> VKPISPEQEELIHRLVYFQNEYEQPSDEDLKRISNTPSEGEDQSDLNFRHITEITILTVQLIVEFAKRLPGFDKLLREDQIALLKACSSEVMMLRMARRYDVGSDSILFANNQPYTRDSYSLAGMGETVDDLLRFCRQMYGMKVDNAEYALLTAIVIFSERPSLIEGWKVEKIQEIYLEALKVYVDNRRKPASGTIFAKLLSVLTELRTLGNLNSEMCFSLKLKNKKLPPFLAEIWDV;> NAVANICQATNSQLYQLVEWAKHIPHFSSLPIEDQVLLLRAGWNELLIAAFSH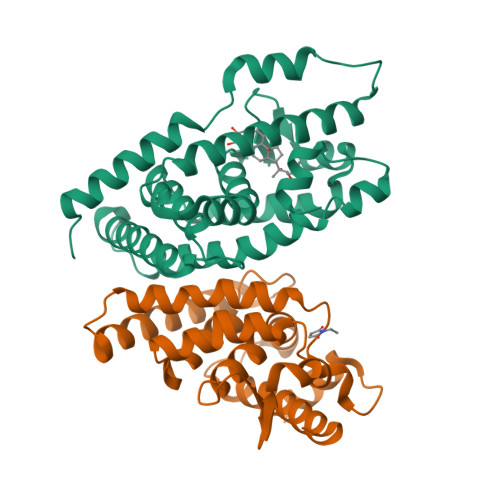RSVEVRDGIVLGAGITVHRNSAHQAGVGTIFDRVLTELVAKMRDMNMDRTELGSLRSIILFNPEVRGLKSGQEVELLREKVYAALEEYTRVTRPEEPGRFAKLLLRLPALRSIGLKCLEHLFFFKLIGDIPIDTFLMDMLGS>TSHHHHHMKKIEHKMVAVNGLNMHLAELGEGPTILFIHGFPELWYSWRHQMVYLAERGYRAVAPDLRGYGDTTGAPLNDPSKFSILHLVGDVVALLEAIAPNEEKVFVVAHDWGALIAWHLCLFRPDKVKALVNLSVHFSKRNPKMNVVEGLKAIYGEDHYISRFQVPGEIEAEFAPIGAKSVLKKILTYRDPAPFYFPKGKGLEAIPDAPVALSSWLSEEELDYYANKFEQTGFTGAVNYYRALPINWELTAPWTGAQVKVP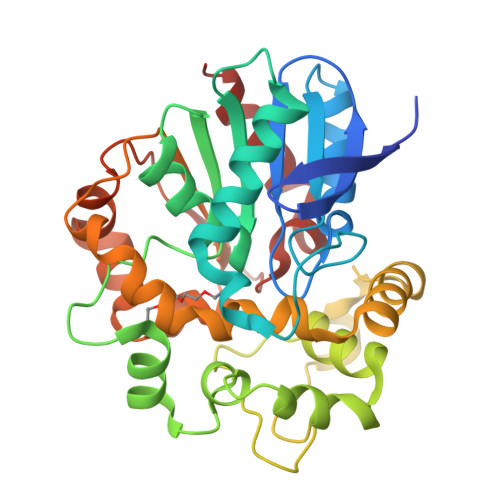TKFIVGEFDLVYHIPGAKEYIHNGGFKKDVPLLEEVVVLEGAAHFVSQERPHEISKHIYDFIQKF[2x]>[2x]DEINKELNQVMEQLGDARIDRQESSRQQRKAEIMESIKRLYPGSVYGRLIDLCQPTQKKYQIAVTKVLGKNMDAIIVDSEKTGRDCIQYIKEQRGEPETFLPLYYLEVKPTDEKLRELKGAKLVIDVIRYEPPHIKKALQYACGNALVCDNVEDARRIAFGGHQRHKTVALDGTLFQKSGVISGGASDLKAKARRWDEK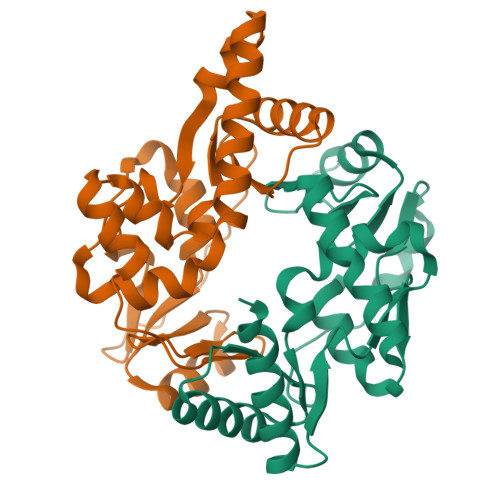AVDKLKEKKERLTEEL;>[2x]AAKREDLEKKQQLLRAATGKAILNGIDSINKVLEHFRRKGINQHVQNGYHGIVMNNFECEPAFYTCVEVTAGNRLFYHIVDSDEVSTKILMEFNKMNLPGEVTFLPLNKLDVRDTAYPETNDAIPMISKLRYNPRFDKAFKHVFGKTLICRSMEVSTQLARAFTMDCITLEGDQVSHRGALTGGYYDTRKSRLELQKDVRKAEEELGELEAKL> 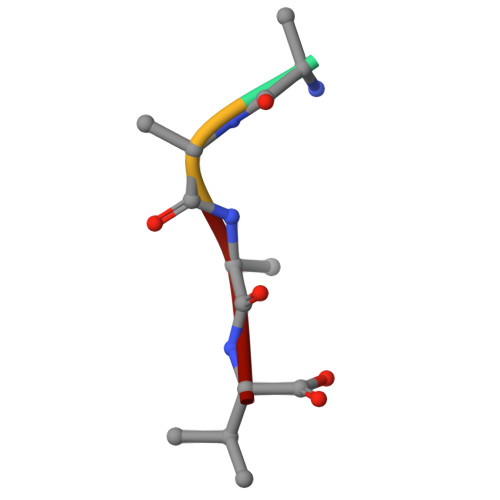AAAV>QTVNARKCSLTGKWTNRMNHNMTIGAVNSRGEFTGTYIATVNATSNEIKESPLHGTQNTIN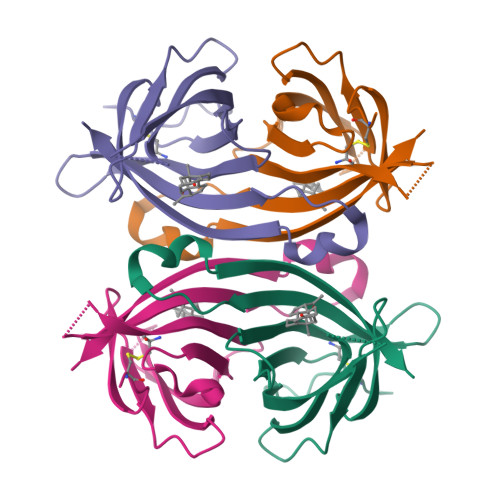KRTQPTFGFTVNWKFSESTTVFTGQCFIDRNGKEVLKTMWLLRSSVNDIGDDWKATRVGYNIFTRLRTQKEHHHHHH[2x]Nucleoside diphosphate kinases (NDPKs) catalyze the reversible transfer of the phosphoryl γ of nucleoside triphosphates to nucleoside diphosphates. The two-step reaction proceeds via a covalent intermediate, the enzyme being transiently phosphorylated on a conserved histidine residue, His117 in Mycobacterium tuberculosis NDPK (Mt-NDPK). Crystal structure of the Mt-NDPK has been solved. It is a hexamer with a tertiary and quaternary structure very similar to other hexameric NDPKs.

One interaction present in Mt-NDPK but missing in other NDPKs, is the intersubunit salt bridge Arg80-Asp93 located on the protein surface. Here, to elucidate the crucial role of that salt bridge for hexamer and overall protein stability, a mutant having the salt bridge abolished (D93N) has been prepared. The aspartate was changed to asparagine since many NDPKs have asparagine in that position. The D93N mutant crystallizes along two different space groups. The two structures are similar (0.40 Å of rmsd for 135 Cα) and differ only slightly in the conformation of αA and α2 helices due to crystal contacts. The overall B-factor values of the two D93N structures (64 Å2 and 71 Å2) are similar and higher than that of the wild type (31 Å2). Analysis of B-factor reveals that (1) two domains, the αA-α2 region (40–70) and the CTerm part (120–136), are highly flexible and (2) the beginning of the Kpn-loop where the mutation is located appears more flexible in the mutant than in the WT structure. The D93N mutant enzymes displayed catalytic properties very similar to those of the wt enzyme, within experimental errors. Replacement of the Asp93 with the neutral asparagine showed a dramatically decrease of the thermal stability. The chemical denaturation studies with urea and GuHCl as denaturants showed a large decrease in hexamer stability as a result of the D93N mutation, while the stability of the isolated subunit was not affected.

> MTERTLVLIKPDGIERQLIGEIISRIERKGLTIAALQLRTVSAELASQHYAEHEGKPFFGSLLEFITSGPVVAAIVEGTRAIAAVRQLAGGTNPVQAAAPGTIRGDFALETQFNLVHGSDSAESAQREIALWFPGA>MNSIQIADETYVAADAARVSAAVADRCSWRRWWPDLRLQVTEDRADKGIRWTVTGALTGTMEIWLEPSMDGVLLHYFLHAEPTGVAAWQLARMNLARMTHHRRV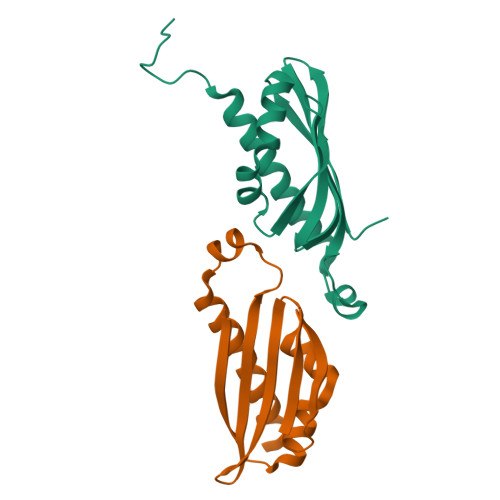AGKKMAFEVKTVLERSRPIGVSPVT[2x]>[2x]MRTRSTISTPNGITWYYEQEGTGPDIVLVPDGLGECQMFDSSVSQIAAQGFRVTTFDMPGMSRSAKAPAETYTEVTAQKLASYVISILDALDIKHATVWGCSSGASTVVALLLGYPDRIR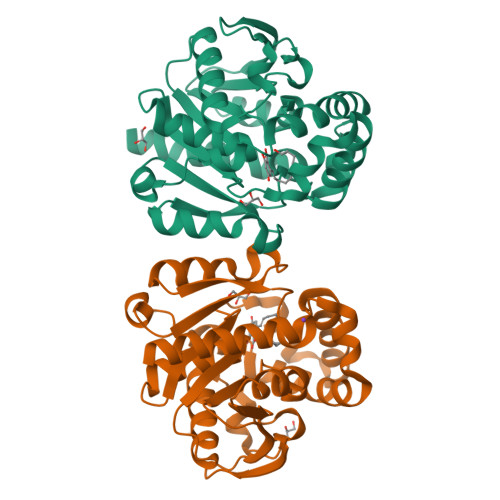NAMCHELPTKLLDHLSNTAVLEDEEISNILANVMLNDVSGGSEAWQALGVEVHARLHKNYPVWARGYPRTIPPSAPVQDVEALRGKPLDWTVGAATPTESFFDNIVTATKAGVNIGLLPGMHFPYVSHPDVFAKYVVETTQKHLWNSSSVDKLAAALEHHHHHH>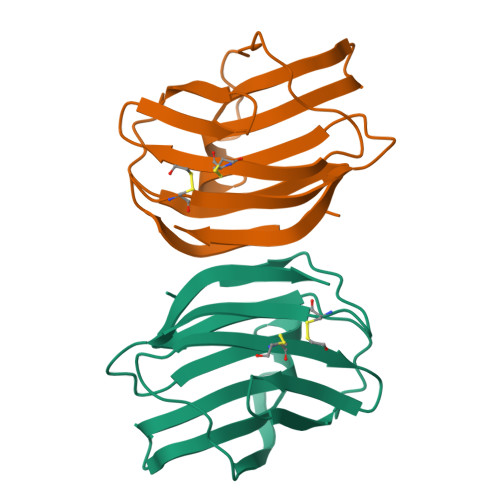[2x]QGLVVTQLDVQPGECVKVKGKILSDAKGFSVNVGKDSSTLMLHFNPRFDCHGDVNTVVCNSKEDGTWGEEDRKADFPFQQGDKVEICISFDAAEVKVKVPEVEFEFPNRLGMEKIQYLAVEGDFKVKAIKFS> MRLRHENKIYKLMCSNCSKEFCKSIYIKKVFSNYMVFDPSVWRFLHVESKRKVSKYLSEDNQPLSDIKCFHCKLDVGRAYKIRGTYLPQLSVKALTFVQESDYSSMTKAKWSDVEQDLFYISEAIEDDFRIMLNALSDTEENIEKKIVLDLDSRQ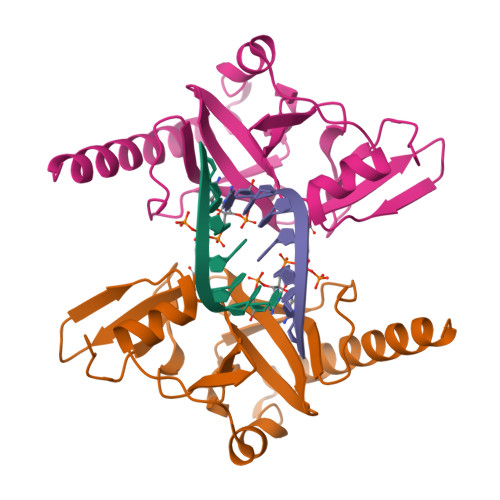HNKQLEMKRFHIQQE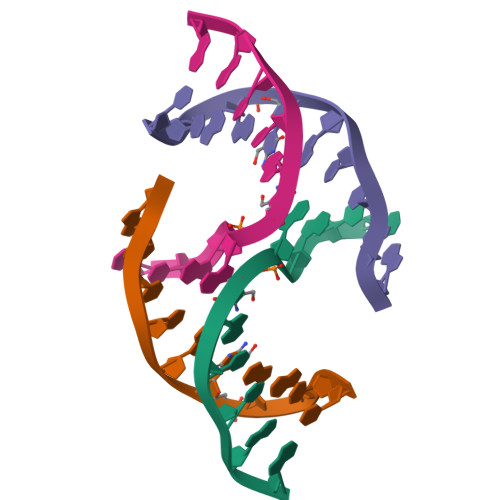>[4x]CCAGXGCTGG3-(carboxymethyl)-4,7-dichloro-1H-indole-2-carboxylic acid 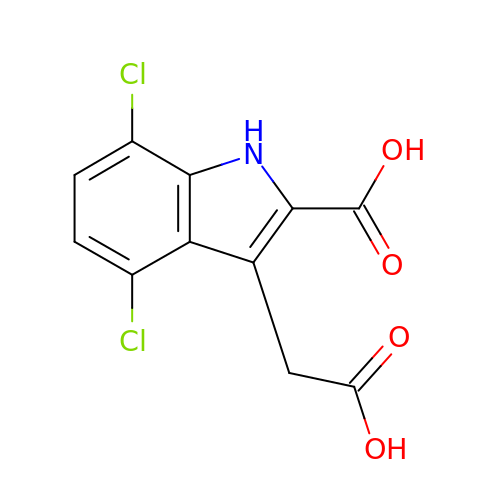| C11 H7 Cl2 N O4 | GQXFZEWSJBOLCT-UHFFFAOYSA-N>GPHSEDEEGQDVTAKVREQEIIRLTQKLITSITTGDYDTYSKLVDPHVTCFEPFSNGNLVEGLEFHKFYFDNTLSKRSVPINTTILSPHVHVLGEDAACICYMRLTQSVNSSGEAKTLQQEETRVWQKKGGNWINVHFHISGKMS[7x]

Ca2+/calmodulin-dependent protein kinase II (CaMKII) is a Ser/Thr kinase that is particularly important in neuronal signaling and cardiac function. CaMKII has a unique architecture, in which the catalytic domains are linked flexibly to a hub domain, also called the association domain, which forms a dodecameric or tetradecameric assembly (see Figure 1A for a description of the domains of CaMKII). We reported recently that the activation of CaMKII-α by ATP and Ca2+/CaM triggers the exchange of activated subunits between different holoenzyme assemblies. Our data are consistent with the idea that the CaM-binding element induces the hub to transition from a closed-ring form to a ring-opened lock-washer configuration, which can release or capture dimer units.

The role of peptide docking in destabilizing the hub emerged from structures of the hubs of two CaMKII isoforms, denoted CaMKII-A and CaMKII-B, present in the sea anemone Nematostella vectensis. N. vectensis, a member of the phylum Cnidaria, is an early branching metazoan. The sequence identity between the hub domains in the two N. vectensis CaMKII isoforms is 62%, and these are 55% and 53% identical to the hub domain of human CaMKII-α respectively. The hub domain of CaMKII-A crystallized at pH 7, while that of CaMKII-B crystallized at pH 4.2. To illustrate this distortion from planarity, we aligned the pH 4.2 N. vectensis CaMKII-B hub structure onto the pH 7.0 CaMKII-A hub structure by superimposing the four subunits that are furthest from the break (E, F, G, and H). We then illustrate the deviation between the two structures with arrows that indicate the displacement of Cα atoms from the flat closed-ring structure (pH 7.0) to the slightly spiral, ring-opened, structure (pH 4.2; the lengths of the arrows are scaled by a factor of 2 for clarity).> GSDDREMDDGRWKASALRVPLQVSSAVIKQEVVTRLAPDPVPLTEGAIGIFLSGTEPESGQEDSGYKVIDNRKYVYSEGHWGPPTANDTIYLVGNDADVCAYYPYKDSYTDKTVIPLQSQDYVETEDIYYALNTMINGFTPAITFDMVHAYSLVELKISRENYFMPCEISKITLKNSNLIKKGTINIAVDGSIHSSETGNYDLTTVTDASPHTLSVGESYVC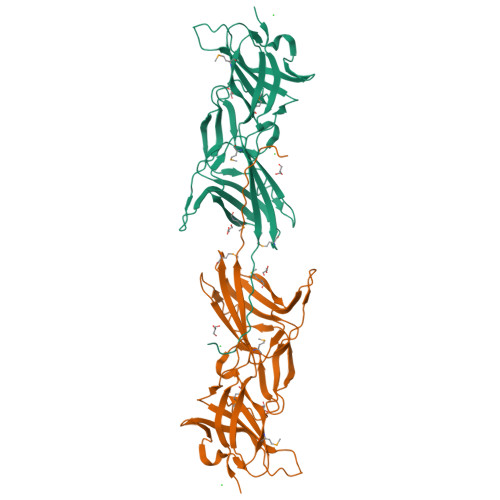RVLMIPVPLKIERTDAEGGEFGLSVSLVIDGQQMLVEIPYSELGEFRQGEKYVIGLKIKGTEIVPTVKALEWEDEEVNGGNKYPVE(2P,2'P)-2,2'-(1,3-phenylene)di(pyridin-4-amine) 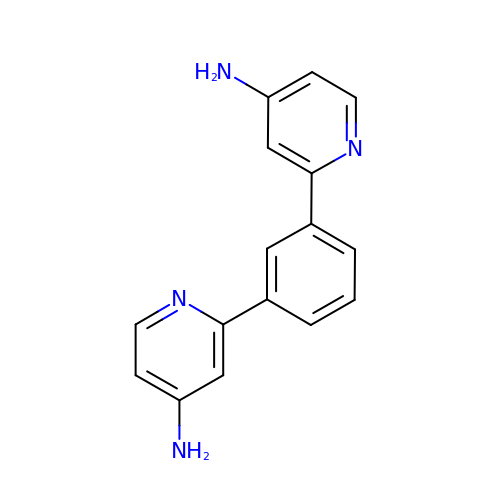| C16 H14 N4 | XLXGLQRJMSGVPH-UHFFFAOYSA-N Cellulose, alginate, the Pel polysaccharide, and poly-β(1,6)-N-acetylglucosamine (PNAG) are each produced by the synthase-dependent pathway. PgaA contains an N-terminal domain with 8 predicted TPR motifs and a C-terminal porin domain, while PgaB is an outer-membrane lipoprotein with an N-terminal de-acetylase (DA) domain and C-terminal glycoside hydrolase (GH) domain. Previous studies have established that PgaA and PgaB form a complex at the outer membrane and that the TPR domain of PgaA is critical for this interaction. Our results suggest a scaffolding role for the TPR domain that combines PNAG/dPNAG translocation with the modulation of its chemical structure by PgaB.

After attempting multiple truncated constructs of the TPR domain (PgaA-32-465, 32–448, 32–431, 32–415, 32–398, 32–382), we found PgaA-32-367 to be the most stable and amenable to crystallization. Diffraction quality crystals were obtained, and the structure was solved using selenomethionine incorporation and the single wavelength anomalous diffraction (SAD) method and refined against a 2.85 Å native dataset. The asymmetric unit contains two molecules (chains A and B), which were modeled from residues 224–359 and 220–343, respectively. There was no remaining unexplained electron density suggesting that the original construct had further fragmented and that only the C-terminal fragment containing residues 220–359 had crystallized. As there is no evidence that PgaA forms a dimer in solution, we presume this domain swap is a crystallization artifact and that only residues 220–342 represent a biologically relevant fold. The structure of PgaA 220–342 is all α-helical and contains TPR-3 and TPR-4, as well as an unusually long α/α-motif containing 46 amino acids that likely represents α/α-5 based on our bioinformatics analysis. The α/α-5 motif differs noticeably from the common TPR fold and locally increases the curvature of PgaA, thus forming a groove with conserved residues on the concave surface of the TPR-like module running parallel to the superhelical axis (groove 1). This increased curvature also results in a groove running diagonal to the superhelical axis on the convex surface with conserved residues from the α/α-5 repeat lining the groove (groove 2). Analysis of the structure revealed that residues lining groove 1 in chains A and chain B are both involved in crystal packing. Combined, these results suggest that dPNAG binds to the conserved groove on the concave TPR surface of residues 220–367 and that W314 and W318 are involved in this interaction.

>DANLTPDIRADIHAELVRLSFMPTRSESERYAIADRALAQYAALEILWHDNPDRTAQYQRIQVDHLGALLTRDRYKDVISHYQRLKKTGQIIPPWGQYWVASAYLKDHQPKKAQSIMTELFYHKETIAPDLSDEELADLFYSHLESEN[2x]> SNAMSKVLVLKSSILATSSQSNQLADFFVEQWQAAHAG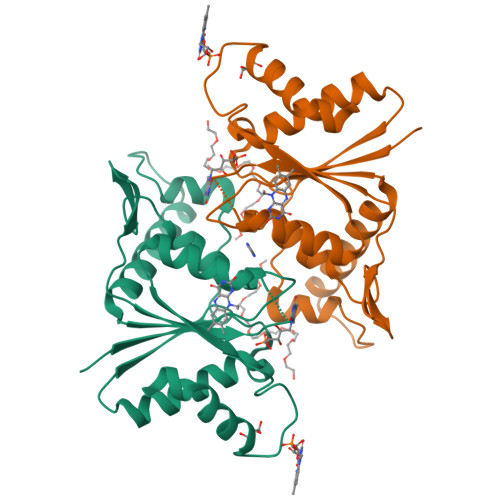DQITVRDLAAQPIPVLDGELVGALRPSGTALTPRQQEALALSDELIAELQANDVIVIAAPMYNFNIPTQLKNYFDMIARAGVTFRYTEKGPEGLVTGKRAIILTSRGGIHKDTPTDLVVPYLRLFLGFIGITDVEFVFAEGIAYGPEVATKAQADAKTLLAQVVAA> GPGYNEPMAASDEVNLIESRTVVPLNTWVLISNFKVAYNILRRPDGTFNRHLAEYLDRKVTANANPVDGVFSFDVLIDRRINLLSRVYRPAYADQEQPPSILDLEKPVDGDIVPVILFFHGGSFAHSSANSAIYDTLCRRLVGLCKCVVVSVNYRRAPENPYPCAYDDGWIALNWVNSRSWLKSKKDSKVHIFLAGDSSGGNIAHNVALRAGESGIDVLGNILLNPMFGGNERTESEKSLDGKYFVTVRDRDWYWKAFLPE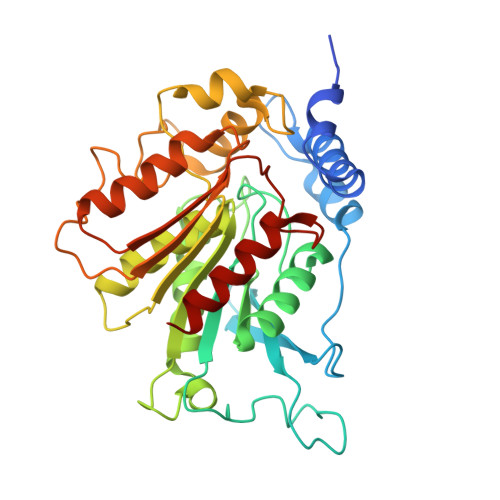GEDREHPACNPFSPRGKSLEGVSFPKSLVVVAGLDLIRDWQLAYAEGLKKAGQEVKLMHLEKATVGFYLLPNNNHFHNVMDEISAFVNAE> GYLVGDAT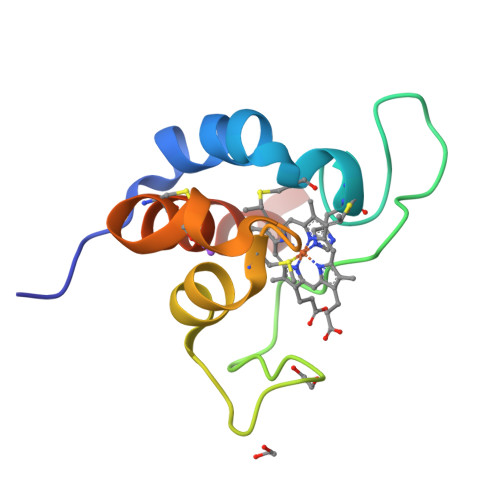RGANLWNTQTCVACHGVDGERNASGTPALTPLNPNRDLYRHSRDTQDRALRDFISMWMPQGNEGSCTGQCAADIEAFIRTWHHHHHH> MATNFDEAVRAKVERPANVPEDRVYEIDMYALNGIEDGYHEAWKKVQHPGIPDLIWTPFTGGHWIATNGDTVKEVYSDPTRFSSEVIFLPKEAGEKAQMVPTKMDPPEHTPYRKALDKGLNLAKIRKVEDKVREVASSLIDSFAARGECDFAAEYAELFPVHVFMALADLPLEDIPVLSEYARQMTRPEGNTPEEMATDLEAGNNGFY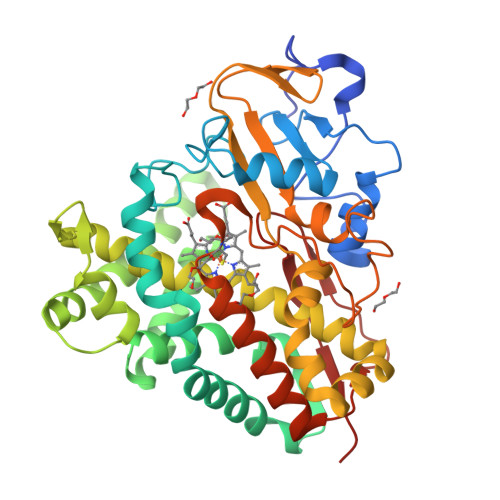AYVDPIIRARVGGDGDDLITLMVNSEINGERIAHDKAQGLISLLLLGGLDTVVNFLSFFMIHLARHPELVAELRSDPLKLMRGAEEMFRRFPVVSEARMVAKDQEYKGVFLKRGDMILLPTALHGLDDAANPEPWKLDFSRRSISHSTFGGGPHRCAGMHLARMEVIVTLEEWLKRIPEFSFKEGETPIYHSGIVAAVENVPLVWPIAR> MKLVTVIIKPFKLEDV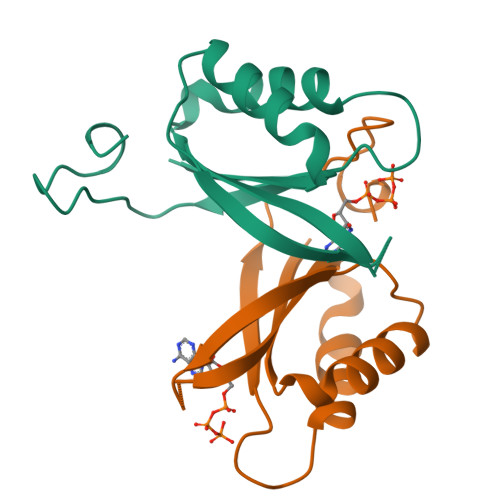REALSSIGIQGLTVTEVKGFGRQKGNAELYRGAEYSVNFLPKVKIDVAIADDQLDEVIDIVSKAAYTGKIGDGKIFVAELQRVIRIRTGEADEAAL>MEIVEYPDPILRAKNKRIDIFDENLKNLVDAMFDVMYKTDGIGLSAPQVGLNVQLMVFNPAGEPGEGKEIVLVNPKIKKYSDKLVPFDEGCLSFPGIYAEVVRPQSVKIDARDITGERFSISLSRLPAR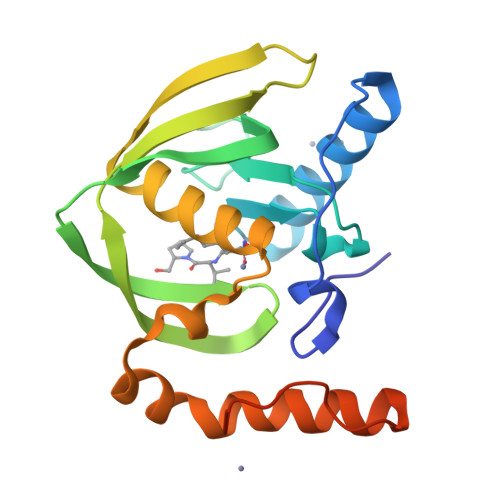IFQHEYDHLEGVLFFDRMTDQVLDSIREELEALEKKYEEKTGLPSPERVEARQKRKAGVGFGKR[2x]>KGTDSLKSSIEKYLKDKKAKVGVAVLGIEDNFKLNVNEKHHYPMQSTYKFHLALAVLDKLDKENISIDKKLFVKKSELLPNTWSPLRDKYPDGNVDLSISEILKATVSRSDNNGCDILFRFVGGTNKVHNFISKLGVKNISIKATEEEMHKAWNVQYTNWTTPDATVQLLKKFYKNEILSKNSYDYLLNTMIETTTGPKRLKGLLPDGTVVAHKTGSSDTNDKGITAATNDIGIITLPNGKHFAIAVYVSDSSEKSDV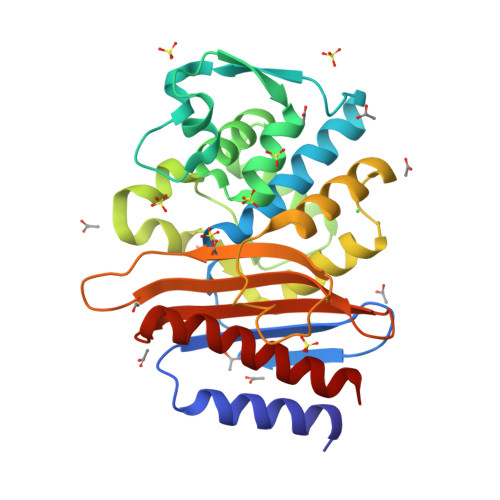NEKIIAEICKSVWDYLVK[4x]>[2x]GKDVITKDMNQLPLPARNFINSNFTKPQVAHIKIDKDMMESTKYEVVLM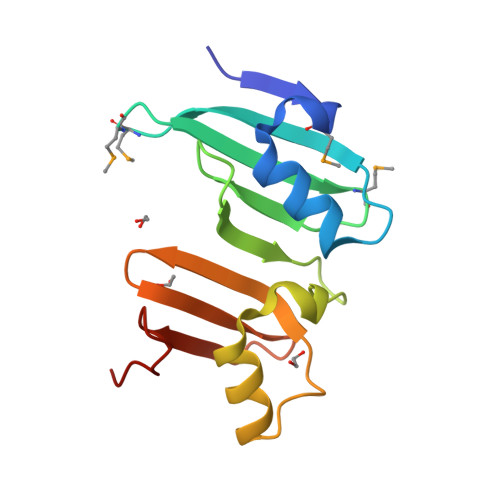DGTEIDFDSKGNWEEVSAKKGQTVPVSIVPGFAVNYLKAHNFVNEGVTKVERDRKGYEIELSTGLSFKFDKKGKFIKTDD>[10x]GAQSEVVVLYPDTENKDLDEAVYQKIFLAGTIDMGKSVDWQKATCDWFRALPEGRYLLF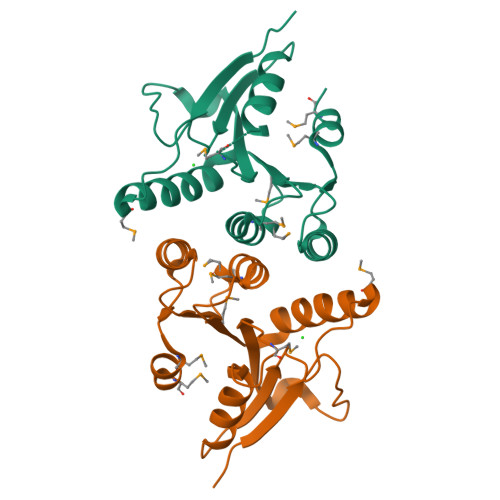NPRRDKGLSGEMSDFEHQVNWELEHLEKADLIIMNILASSKSPITLLEMGLFMRSGKLRVICEPGFYRYDNVRLTCARYGVPLYQNMDDFLKTMR> AYPSFEAYSNYKVDRTDLETFLDKQKEVSLYYLLQNIAYPEGQFNNGVPGTVIASPSTSNPDYYYQWTRDSAITFLTVLSELEDNNFNTTLAKAVEYYINTSYNLQRTSNPSGSFDDENHKGLGEPKFNTDGSAYTGAWGRPQNDGPALRAYAISRYLNDVNSLNEGKLVLTDSGDINFSSTEDIYKNIIKPDLEYVIGYWDSTGFDLWEENQGR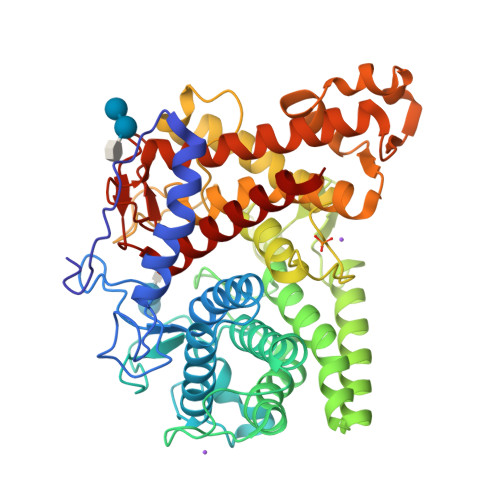HFFTSLVQQKALAYAVDIAKSFDDGDFANTLSSTASTLESYLSGSDGGFVNTDVNHIVENPDLLQQNSRQGLDSATYIGPLLTHDIGESSSTPFDVDNEYVLQSYYLLLEDNKDRYSVNSAYSAGAAIGRYPEDVYNGDGSSEGNPWFLATAYAAQVPYKLAYDAKSASNDITINKINYDFFNKYIVDLSTINSAYQSSDSVTIKSGSDEFNTVADNLVTFGDSFLQVILDHINDDGSLNEQLNRYTGYSTGAYSLTWSSGALLEAIRLRNKVKALA> MIGVNIYLLLIGVATLLSMYRVFRGPTTVDRLVAVDIMTTITVGLMVLFALYYRRIIFLDVALVYAILSFAGVIA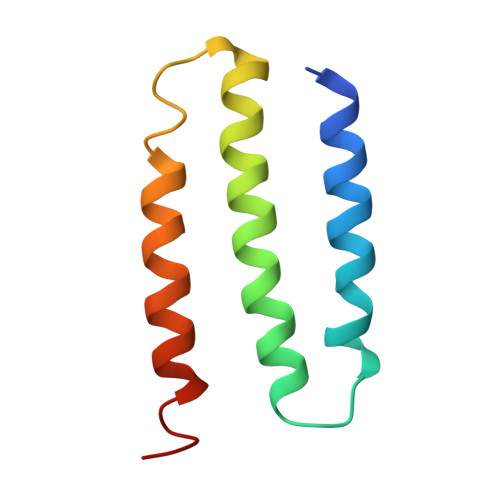FARYLEGGL(5-(PYRIDIN-3-YL)FURAN-2-YL)METHANAMINE | C10 H10 N2 O | 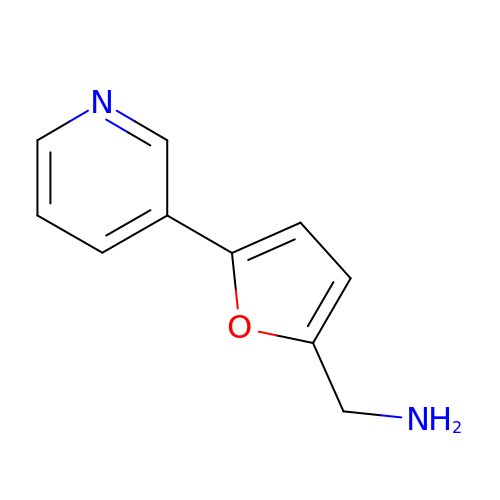LENAVORGWBTPJR-UHFFFAOYSA-N(2~{S})-3-azanyl-2-[[(2~{S})-4-methyl-2-[[oxidanyl(phenylmethoxycarbonylaminomethyl)phosphoryl]amino]pentanoyl]amino]propanoic 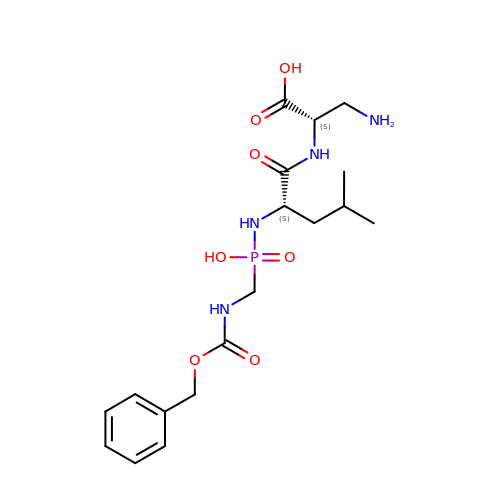acid | C18 H29 N4 O7 P | XMQOUWSDXLWVTQ-GJZGRUSLSA-N>[2x]ARSTDTFNYATYHTLEEIYDFLDLLVAENPHLVSKIQIGNTYEGRP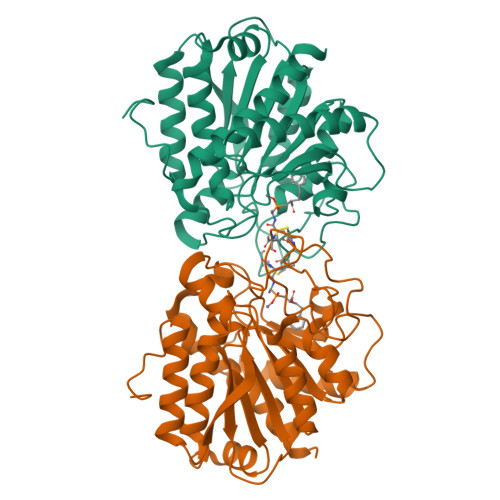IYVLKFSTGGSKRPAIWIDTGIHSREWVTQASGVWFAKKITQDYGQDAAFTAILDTLDIFLEIVTNPDGFAFTHSTNRMWRKTRSHTAGSLCIGVDPNRNWDAGFGLSGASSNPCSETYHGKFANSEVEVKSIVDFVKDHGNIKAFISIHSYSQLLMYPYGYKTEPVPDQDELDQLSKAAVTALASLYGTKFNYGSIIKAIYQASGSTIDWTYSQGIKYSFTFELRDTGRYGFLLPASQIIPTAKETWLALLTIMEHTLNHPY> MRI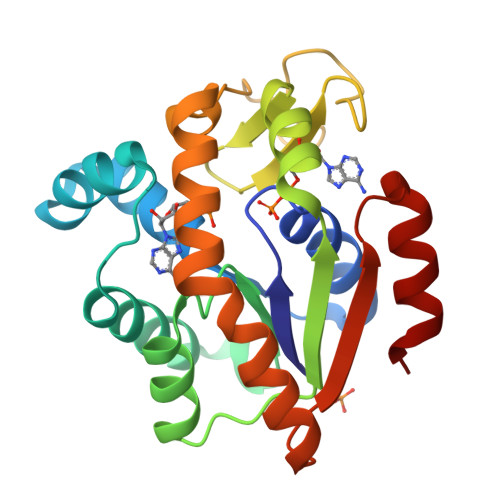ILLGAPGAGKGTQAQFIMAKFGIPQISTGDMLRAAIKAGTELGKQAKSVIDAGQLVSDDIILGLVKERIAQDDCAKGFLLDGFPRTIPQADGLKEVGVVVDYVIEFDVADSVIVERMAGRRAHLASGRTYHNVYNPPKVEGKDDVTGEDLVIREDDKEETVLARLGVYHNQTAPLIAYYGKEAEAGNTQYLKFDGTKAVAEVSAELEKALA> KTTQSTL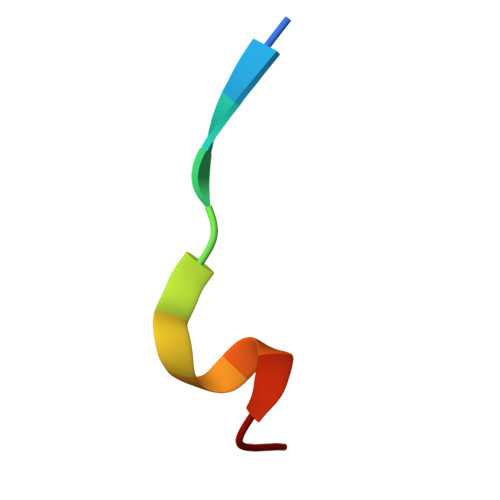DSFFK1-cyclohexyl-3-[[(2~{R})-oxolan-2-yl]methyl]urea 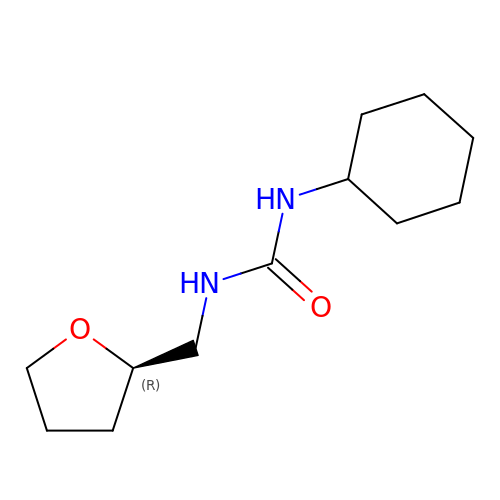| C12 H22 N2 O2 | RYUZWZOTJULRNS-LLVKDONJSA-N>[8x]MG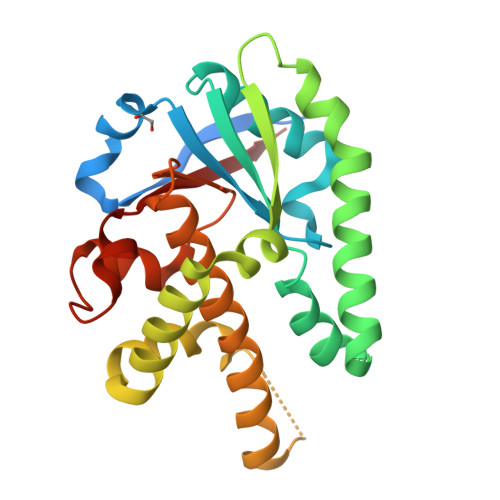HHHHHHGEPREEPAKPVFGRRYKAEIGSVSPTTSRDTFEDHDTCFLGVSLENSNFKPAKVDAMAKWISRRFSQCTVLIGDSIHRITLESTRSMPPRAALDDALRLGREFVESRQPVFESFRDRTKFTFVTCSEVQSWGLYGDYHERLRQHYDQDAAFRGSVEAFGRDYHGKRSEGVSAQELDHRIRKSSEYFLEEFAIFACLQRTGSPVMVYPGSFSTLSEIAQGKHPGAPEELRDLIVVSLHLKGR> MACWPQLRLLLWKNLTFRRRQTCQLLLEVAWPLFIFLILISVRLSYPPYEQHECHFPNKAMPSAGTLPWVQGIICNANNPCFRYPTPGEAPGVVGNFNKSIVARLFSDARRLLLYSQKDTSMKDMRKVLRTLQQIKKSSSNLKLQDFLVDNETFSGFLYHNLSLPKSTVDKMLRADVILHKVFLQGYQLHLTSLCNGSKSEEMIQLGDQEVSELCGLPREKLAAAERVLRSNMDILKPILRTLNSTSPFPSKELAEATKTLLHSLGTLAQELFSMRSWSDMRQEVMFLTNVNSSSSSTQIYQAVSRIVCGHPEGGGLKIKSLNWYEDNNYKALFGGNGTEEDAETFYDNSTTPYCNDLMKNLESSPLSRIIWKALKPLLVGKILYTPDTPATRQVMAEVNKTFQELAVFHDLEGMWEELSPKIWTFMENSQEMDLVRMLLDSRDNDHFWEQQLDGLDWTAQDIVAFLAKHPEDVQSSNGSVCTWREAFNETNQAIRTISRFMECVNLNKLEPIATEVWLINKSMELLDERKFWAGIVFTGITPGSIELPHHVKYKIRMDIDNVERTNKIKDGYWDPGPRADPFEDMRYVWGGFAYLQDVVEQAIIRVLTGTEKKTGVYMQQMPYPCYVDDIFLRVMSRSMPLFMTLAWIYSVAVIIKGIVYEKEARLKETMRIMGLDNSILWFSWFISSLIPLLVSAGLLVVILKLGNLLPYSDPSVVFVFLSVFAVVTILQCFLISTLFSRANLAAACGGIIYFTLYLPYVLCVAWRDYVGFTLKIFASLLSPVAFGFGCEYFALFEEQGIGVQWDNLFESPVEEDGFNLTTSVSMMLFDTFLYGVMT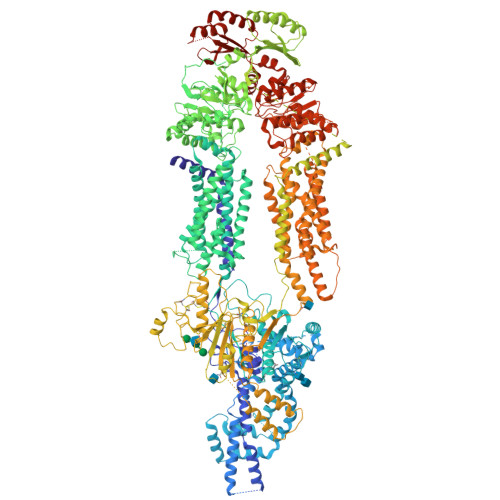WYIEAVFPGQYGIPRPWYFPCTKSYWFGEESDEKSHPGSNQKRISEICMEEEPTHLKLGVSIQNLVKVYRDGMKVAVDGLALNFYEGQITSFLGHNGAGKTTTMSILTGLFPPTSGTAYILGKDIRSEMSTIRQNLGVCPQHNVLFDMLTVEEHIWFYARLKGLSEKHVKAEMEQMALDVGLPSSKLKSKTSQLSGGMQRKLSVALAFVGGSKVVILDEPTAGVDPYSRRGIWELLLKYRQGRTIILSTHHMDEADVLGDRIAIISHGKLCCVGSSLFLKNQLGTGYYLTLVKKDVESSLSSCRNSSSTVSYLKKEDSVSQSSSDAGLGSDHESDTLTIDVSAISNLIRKHVSEARLVEDIGHELTYVLPYEAAKEGAFVELFHEIDDRLSDLGISSYGISETTLEEIFLKVAEESGVDAETSDGTLPARRNRRAFGDKQSCLRPFTEDDAADPNDSDIDPESRETDLLSGMDGKGSYQVKGWKLTQQQFVALLWKRLLIARRSRKGFFAQIVLPAVFVCIALVFSLIVPPFGKYPSLELQPWMYNEQYTFVSNDAPEDTGTLELLNALTKDPGFGTRCMEGNPIPDTPCQAGEEEWTTAPVPQTIMDLFQNGNWTMQNPSPACQCSSDKIKKMLPVCPPGAGGLPPPQRKQNTADILQDLTGRNISDYLVKTYVQIIAKSLKNKIWVNEFRYGGFSLGVSNTQALPPSQEVNDAIKQMKKHLKLAKDSSADRFLNSLGRFMTGLDTKNNVKVWFNNKGWHAISSFLNVINNAILRANLQKGENPSHYGITAFNHPLNLTKQQLSEVALMTTSVDVLVSICVIFAMSFVPASFVVFLIQERVSKAKHLQFISGVKPVIYWLSNFVWDMCNYVVPATLVIIIFICFQQKSYVSSTNLPVLALLLLLYGWSITPLMYPASFVFKIPSTAYVVLTSVNLFIGINGSVATFVLELFTDNKLNNINDILKSVFLIFPHFCLGRGLIDMVKNQAMADALERFGENRFVSPLSWDLVGRNLFAMAVEGVVFFLITVLIQYRFFIRPRPVNAKLSPLNDEDEDVRRERQRILDGGGQNDILEIKELTKIYRRKRKPAVDRICVGIPPGECFGLLGVNGAGKSSTFKMLTGDTTVTRGDAFLNKNSILSNIHEVHQNMGYCPQFDAITELLTGREHVEFFALLRGVPEKEVGKVGEWAIRKLGLVKYGEKYAGNYSGGNKRKLSTAMALIGGPPVVFLDEPTTGMDPKARRFLWNCALSVVKEGRSVVLTSHSMEECEALCTRMAIMVNGRFRCLGSVQHLKNRFGDGYTIVVRIAGSNPDLKPVQDFFGLAFPGSVLKEKHRNMLQYQLPSSLSSLARIFSILSQSKKRLHIEDYSVSQTTLDQVFVNFAKDQSDDDHLKDLSLHKNQTVVDVAVLTSFLQDEKVKESYVGDYKDDDDK>[2x]GSHMMAEQVALSRTQVCGILREELFQGDAFHQSDTHIFIIMGASGDLAKKKIYPTIWWLFRDGLLPENTFIVGYARSRLTVADIRKQSEPFFKATPEEKLKLEDFFARNSYVAGQYDDAASYQRLNSHMNALHLGSQANRLFYLALPPTVYEAVTKNIHESCMSQIGWNRIIVEKPFGRDLQSSDRLSNHISSLFREDQIYRIDHYLGKEMVQNLMVLRFANRIFGPIWNRDNIACVILTFKEPFGTEGRGGYFDEFGIIRDVMQNHLLQMLCLVAMEKPCSTNSDDVRDEKVKVLKCISEVQANNVVLGQYVGNPDGEGEATKGYLDDPTVPRGSTTATFAAVVLYVENERWDGVPFILRCGKALNERKAEVRLQFHDVAGDIFHQQCKRNELVIRVQPNEAVYTQMMTKKPGMFFNPEESELDLTYGNRYKNVKLPDAYERLILDVFCGSQMHFVRSDELREAWRIFTPLLHQIELEKPKPIPYIYGSRGPTEADELMKRVGFQYEGTYKWVNPHKLC

pmcGlucose-6-phosphate dehydrogenase (G6PD) is a housekeeping enzyme that generates NADPH. G6PD exists as a monomer, homodimer, and homotetramer, with each monomer having three binding sites: one for catalytic glucose-6-phosphate (G6P), one for an NADP+ cofactor, and an allosteric NADP+-binding site. The latter allosteric NADP+-binding site, also known as the structural NADP+-binding site, is important for maintaining long-term protein stability and for promoting oligomer assembly. Oligomerization is central to G6PD function as it controls the activity of G6PD; the monomer is inactive with both the dimer and tetramer being the active forms.

As G6PDK403Q has been established as a good model for Class I variants, we sought to determine if stabilizing the dimer or tetramer could correct activity or stability for G6PDK403Q. Using the same mutagenic strategy described above, we made double and triple mutants, the G6PDK403Q mutation combined with either dL, or both dL and tetramer-locked (tL), to determine if inducing oligomerization could recover activity and/or stability for G6PDK403Q. In contrast, locking G6PDK403Q in the tetrameric state improved activity significantly, ∼200-fold. Consistent with the fact that tetramer locking was able to activate G6PDK403Q, G6PDK403QdLtL improved G6P and NADP+ binding significantly, as the Km changed from 1382 to 102 μM for G6P and from 802 to 59 μM for NADP+. When examining protein stability, both dimer and tetramer locking improved G6PDK403Q stability; dimer locking increased protein stability by 2.0 °C with tetramer locking further increasing stability by 3.9 °C, bringing G6PDK403QdLtL thermostability to that of G6PDWT. When running G6PDK403Q and G6PDK403QdLtL on SEC in monomer conditions, up to 80% of G6PDK403QdLtL was a tetramer, confirming that the G6PDK403QdLtL mutant can form a tetramer. Interestingly, the G6PDK403QdLtL dimer recovered the missing ßM strand of the structural NADP+ ß-sheet, lost in G6PDK403Q. Additionally, the globular shape of the dimer is modified, with a hinge-like shift in one of the monomers relative to the other monomer in the dimer (salmon to teal). This shift is illustrated using G341 as a reference point; there is a 39.6 Å and 55.3 Å distance between monomers of G6PDK403Q and G6PDK403QdLtL, respectively, and the catalytic NADP+ site is shifted by 20.4 Å. As A277C is located at opposing ends of the αj-helix, tetramer locking through disulfide bond formation likely prevents the αj-helix from shifting, which maintains the K290/E287 and E347/K275 salt bridges, reducing shifting of the structural NADP+ ß-sheet.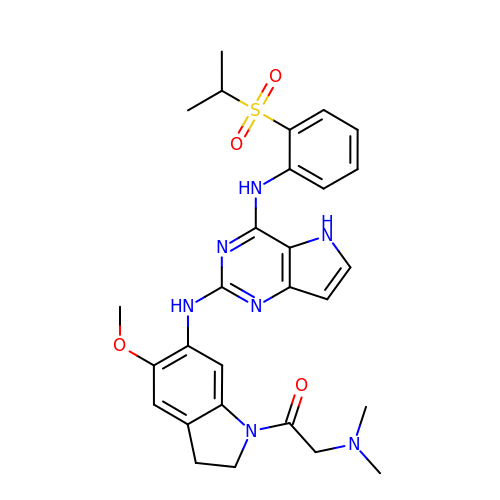2-(dimethylamino)-1-[5-methoxy-6-[[4-[(2-propan-2-ylsulfonylphenyl)amino]-5H-pyrrolo[3,2-d]pyrimidin-2-yl]amino]-2,3-dihydroindol-1-yl]ethanone | C28 H33 N7 O4 S | HTWIYZGXLMTRHE-UHFFFAOYSA-N> STNDLETAGGAELTTHSSHYLVQGDNSSGISDDFEPKEFILTDNEMEQITNEMERNHLDYLRNSKQVQSQLQTLRSEIAPHKIEENQSNLDILSEAQIKAGENK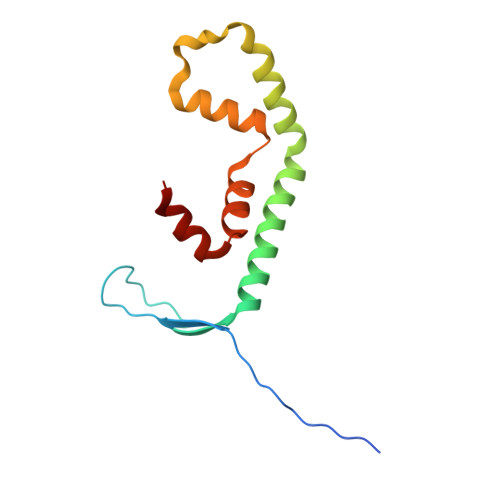YSTLKKLKSGSTKARVAFFEEL>[6x]MKTQIINGVSLPNIPWQDKPADCKDVIWRYDANPIIPRDQLPTSNSIFNSAVVPYESEKGKFAGVFRVDDKCRNMELHAGFSKDGIHWDINPDRIVFEQAEKSTEEVNQWGYGYDPRVCFIEDRFWVTWCNAYGWK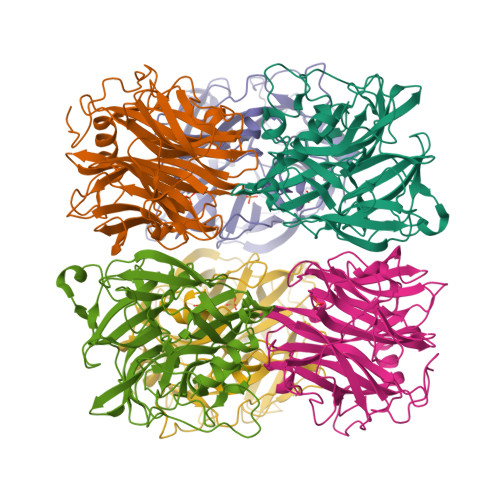PTIGVAYTFDFKTFYQCENAFLPFNRNGVLFPRKINGKYVMFSRPSDSGHTPFGDMFISQSPDMKYWGEHRHVMGPLRAWESKKIGAGPIPIETSEGWLCFYHGVLESCNGFVYSFSACILDKDEPWKVKYRCAEYLLSPQKIYECVGDVQNVTFPCATLVDADTGRIAIYYGCADTCVSMAFTTVDDVVDYVKSHSSV We also solved the crystal structure of BmTrxR, being the first crystallographic structure of a TrxR from a nematode, which, surprisingly, is a fusion of a large TrxR domain with a Grx-like domain at the N-terminus lacking a typical Grx active site motif. Helminth TrxRs are members of the high molecular weight TrxR subfamily and are selenocysteine (Sec, U)-containing homodimeric flavoenzymes. They transfer reducing equivalents from NADPH to their flavin adenine dinucleotide (FAD) cofactor and, subsequently, to a pair of cysteines located at the si-face of the isoalloxazine ring. From there, electrons are transferred to the mobile Sec-containing C-terminal redox center of the symmetrical subunit, that, upon reduction of its Cys-Sec motif, reaches the solvent-exposed surface of the enzyme transferring electrons to the incoming oxidized Trx.

Expressing isoform D of BmTrxR, containing the shortest N-terminal extension with respect to the TrxR and Grx domains that are identical in all three isoforms and utilizing a more recent method for Sec insertion capable of yielding 95–100% of the wild-type form, resulted in a protein producing crystals diffracting up to ∼2.5 Å in C212121 space group. Upon model building, BmTrxR appears to be a fusion of a Grx-like domain (14–102) with a TrxR domain (103–598), reminiscent of the W-shape architecture found in TGR from platyhelminths. Protein dimerization takes place through the TrxR domain, while the Grx domains lie in the upper external arms of the “W”. There are 3 protein subunits in the asymmetric unit of the crystal lattice; 2 of the 3 subunits, subunit a and b, belong to a physiological dimer while the third, subunit c, forms a physiological dimer with a symmetry-related subunit belonging to an adjacent unit cell. Unusually for this class of proteins, the last four residues of the Sec-containing C-terminus are here visible in the electron density, thanks to a particular arrangement of BmTrxR subunits in the crystal lattice. The last four residues (-GCUG) of subunit b have been detected in the X-ray derived electron density because they are trapped between subunit a and subunit c belonging to an adjacent unit cell by a disulfide bridge (2.05 Å) between C596(b)-C22(a) and a selenenylsulfide bond (2.1 Å) between U597(b)-C22(c), respectively. Three cysteines are found in this domain, C22, C82 and C83. While the last two residues are buried, C22 is exposed toward the TrxR domain, about 30 Å apart from the last visible residue of the C-terminus of the TrxR domain of the parent subunit [C22a(CA) - E586b(CA) = 29 Å]. C22 is likely to be a low pKa Cys; it localizes just at the top of an α-helix belonging to the TrxR domain of the same subunit making polar interactions with the carbonyls of F456 and L455 at the top of this helix (the sulfur atom is at 3.4 Å and 3.8 Å from the two oxygens, respectively) and it is within 6.0 Å of the positively charged nitrogens of Arg251 and Lys130 side chains.

>MSPIPNRVSSGSLADAVFKSACEERILLAYADYNPDMTKVVNLFSKYNETVNTVRVSNDAVKDILEIVGWPSMPLIFVKGNCCGGFKELYQLEESGFLNEWLKEHEYDLAIVGGGSGGLAAAKEAVRLGKKVVCLDFVKPSAMGTTWGLGGTCVNVGCIPKKLMHQAALLGEYIEDAKKFGWEIPEGAIKLNWHQLKNAVQNHIASLNWGYRVQLKEKSVTYMNSYATFTGSHELSVKNKKGKVEKVTADRFLIAVGLRPRFPDVPGALECCISSDDLFSLPYNPGKTLCVGASYVSLECAGFLKGIGNDVTVMVRSVLLRGFDQDMAERIKKHMTERGVKFVQCVPIKYERLKKPTDSEPGMIRVHTMQEDEDGTKEVTEDFNTVLMAIGRDAMTDDLGLDVVGVNRAKSGKIIGRREQSVSCPYVYAIGDVLYGSPELTPVAIQAGKVLMRRLFTGSSELTEYDKIPTTVFTPLEYGSCGLSEYSAIQKYGKENINVYHNVFIPLEYAVTERKEKTHCYCKLICLKNEQDLILGFHILTPNAGEITQGFAIALKFDAKKADFDRLIGIHPTVAENFTTLTLVKEDGQTLKATGCUG[3x]>[6x]MIQGVIQKIAGPAVIAKGMLGARMYDICKVGEEGLVGEIIRLDGDTAFVQVYEDTSGLKVGEPVVSTGLPLAVELGPGMLNGIYDGIQRPLERIREKTGIYITRGVVVHALDREKKWAWTPMVKPGDEVRGGMVLGTVPEFGFTHKILVPPDVRGRVKEVKPAGEYTVEEPVVVLEDGTELKMYHTWPVRRARPVQRKLDPNTPFLTGMRILDVLFPVAMGGTAAIPGPFGSGKTVTQQSLAKWSNADVVVYVGCGERGNEMTDVLVEFPELTDPKTGGPLMHRTVLIANTSNMPVAAREASIYVGVTIAEYFRDQGFSVALMADSTSRWAEALREISSRLEEMPAEEGYPPYLAARLAAFYERAGKVITLGGEEGAVTIVGAVSPPGGDMSEPVTQSTLRIVGAFWRLDASLAFRRHFPAINWNGSYSLFTSALDPWYRENVAEDYPELRDAISELLQREAGLQEIVQLVGPDALQDAERL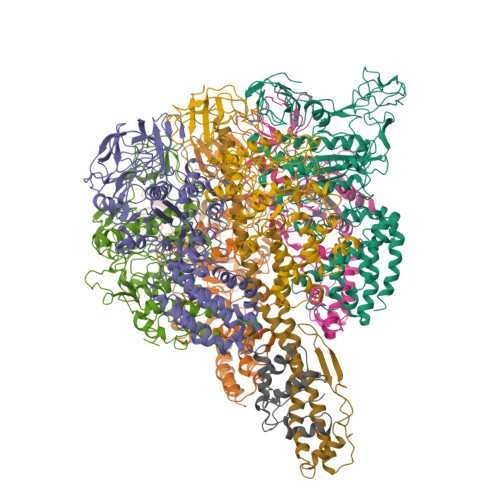VIEVGRIIREDFLQQNAYHEVDAYCSMKKAYGIMKMILAFYKEAEAAIKRGVSIDEILQLPVLERIGRARYVSEEEFPAYFEEAMKEIQGAFKAL;>[6x]EYTGITYISGPLLFVENAKDLAYGAIVDIKDGTGRVRGGQVIEVSEEYAVIQVFEETTGLDLATTSVSLVEDVARLGVSKEMLGRRFNGIGKPIDGLPPITPEKRLPITGLPLNPVARRKPEQFIQTGISTIDVMNTLVRGQKLPIFSGSGLPANEIAAQIARQATVRPDLSGEGEKEEPFAVVFAAMGITQRELSYFIQEFERTGALSRSVLFLNKADDPTIERILTPRMALTVAEYLAFEHDYHVLVILTDMTNYCEALREIGAAREEIPGRRGYPGYMYTDLATIYERAGVVEGKKGSVTQIPILSMPDDDRTHPIPDLTGYITEGQIQLSRELHRKGIYPPIDPLPSLSRLMNNGVGKGKTREDHKQVSDQLYSAYANGVDIRKLVAIIGEDALTENDRRYLQFADAFERFFINQGQQNRSIEESLQIAWALLSMLPQGELKRISKDHIGKYY;>[2x]SQVSPTRMNLLQRRGQLRLAQKGVDLLKKKRDALVAEFFGLVREAMEARKALDQAAKEAYAALLLAQAFDGPEVVAGAALGVPPLEGVEAEVENVWGSKVPRLKATFPDGALLSPVGTPAYTLEASRAFRRYAEALIRVANTETRLKKIGEEIKKTTRRVNALEQVVIPGIRAQIRFIQQVLEQREREDTFRLKRIKGKIEAREAEEEGG;>MAVIADPETAQGFRLAGLEGYGASSAEEAQSLLETLVERGGYALVAVDEALLPDPERAVERLMRGRDLPVLLPIAGLKEAFQGHDVEGYMRELVRKTIGF[2x]> GSHMNGHIYAVGGYDGHTHLNSVEAYDPETDEWRLVAPLTTPRSGMGVAVLNGHIYAVGGYDGHTHLNSVEAYDPETDEWRLVAPLTTPRSGMGVAVLNGHIYAVGGYDGHTHLNSVEAY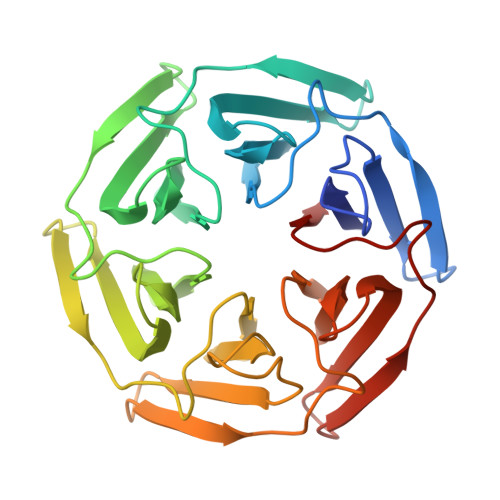DPETDEWRLVAPLTTPRSGMGVAVLNGHIYAVGGYDGHTHLNSVEAYDPETDEWRLVAPLTTPRSGMGVAVLNGHIYAVGGYDGHTHLNSVEAYDPETDEWRLVAPLTTPRSGMGVAVLNGHIYAVGGYDGHTHLNSVEAYDPETDEWRLVAPLTTPRSGMGVAVL>[6x]MAHHHHHHGTEKTPDDVFKLAKDEKVEYVDVRFCDLPGIMQHFTIPASAFDKSVFDDGLAFDGSSIRGFQSI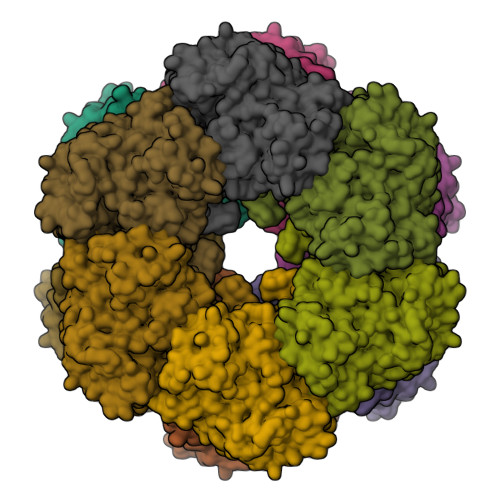HESDMLLLPDPETARIDPFRAAKTLNINFFVHDPFTLEPYSRDPRNIARKAENYLISTGIADTAYFGAEAEFYIFDSVSFDSRANGSFYEVDAISGWWNTGAATEADGSPNRGYKVRHKGGYFPVAPNDQYVDLRDKMLTNLINSGFILEKGHHEVGSGGQAEINYQFNSLLHAADDMQLYKYIIKNTAWQNGKTVTFMPKPLFGDNGSGMHCHQSLWKDGAPLMYDETGYAGLSDTARHYIGGLLHHAPSLLAFTNPTVNSYKRLVPGYEAPINLVYSQRNRSACVRIPITGSNPKAKRLEFRSPDSSGNPYLAFSAMLMAGLDGIKNKIEPQAPVDKDLYELPPEEAASIPQTPTQLSDVIDRLEADHEYLTEGGVFTNDLIETWISFKRENEIEPVNIRPHPYEFALYYDV>MGSHHHHHHHHENLYFQSFETATNAVKNMGVGWNLGNTLDANDATKTWTTTVQHETCWGQPVTKPELFKMMKEAGFGAIRVPVTWYQEMDANGKVNEAWMKRVKEVVDYVVAQDMYCIINVHHDTGADKDAFKSWIKADEANYNQNKAKYEYLWRQIAEAFKDYGDKVLFESYNEMLDKLNSWCFASFAASGQYDATVATSAYNAINGYARSFVNAVRGTGGNNVRRNLIVNTYAAANGSGNWNAHLKDPLSKLVIPQGERDHIAVQVHAYPTIAGKTISAIRTDTRDLMNGLNTYFVSKGIPVIIGEWSTSNVDAKETDYDARKSLMFQFVDDFVAQAKALGI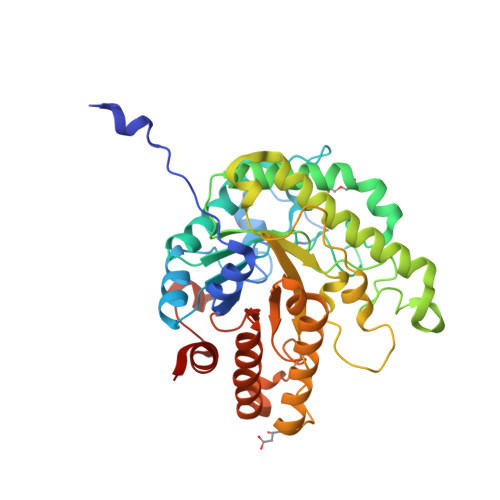ATFYWMGLSDGASRTMPSFNQADLAERIAKAYHGV[2x]> MKLKSFGVFGNPIKHSKSPLIHNACFLTFQKELRFLGHYHPI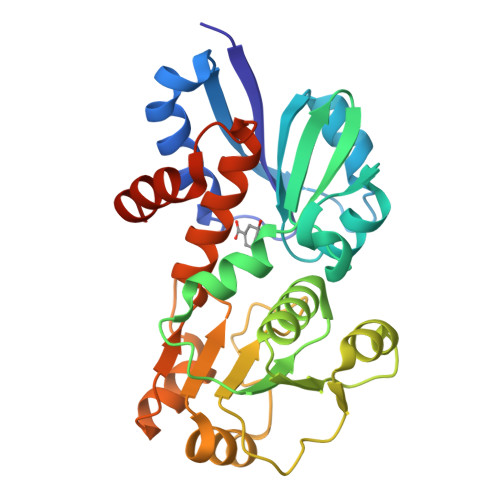LLPLESHIKSEFLHLGLSGANVTLPFKERAFQVCDKIKGIALECGAVNTLVLENDELVGYNTDALGFYLSLKQKNYQNALILGAGGSAKALACELKKQGLQVSVLNRSSRGLDFFQRLGCDCFMEPPKSAFDLIINATSASLHNELPLNKEVLKGYFKEGKLAYDLAYGFLTPFLSLAKELKTPFQDGKDMLIYAAALSFEKFSASQIPYSKAFEVMRSVFLEHHHHHH>MSDYNYKPTLWTRADALKVHEDDPTTTQPVIDIAFPVMSEEVFIWDTMPLRDFDGEIISVNGWCIIFTLTADRNTDNPQFQDENGNYDITRDWEDRHGRARICYWYSRTGKDWIFGGRVMAEGVSPTTREWAGTPILLNDRGDIDLYYTCVTPGATIAKVRGKIVTSDQSVSLEGFQQVTSLFSADGTIYQTEEQNAFWNFRDPSPFIDRNDGKLYMLFEGNVAGPRGSHEITQAEMGNVPPGYEDVGGAKYQAGCVGLAVAKDLSGSEWQILPPLITAVGVNDQTERPHFVFQDGKYYLFTISHKYTFADNLTGPDGVYGFVSDKLTGPYTPMNSSGLVLGNPSSQPFQTYSHYVMPNGLVTSFIDSVPWKGKDYRIGGTEAPTVKILL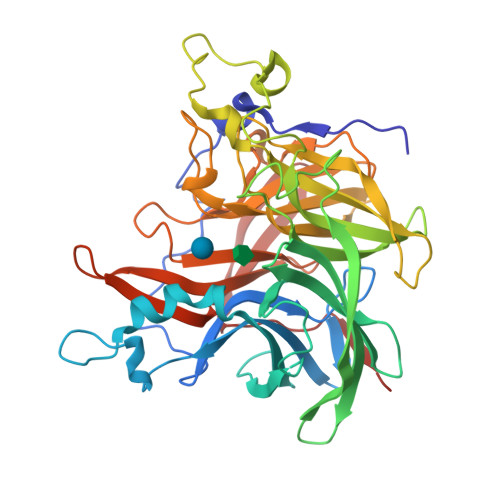KGDRSFIVDSFDYGYIPAMKDITLK[8x]In some pathogenic microbes, the response to oxidative stress is controlled by a SirTM/zinc-containing macrodomain (Zn-Macro) pair responsible for establishment and removal of the modification, respectively. Strikingly, however, the “catalytic loop” found in all other MacroD-type enzymes (also termed “loop 1”) is replaced with and extended loop containing the zinc-coordinating Cx(4)HxC motif, here termed the Zn-loop. To gain a closer understanding of the functional role of the 3α-bundle and coordinated Zn2+ ion, we solved structures from the three sub-branches of Zn-Macros namely from S. aureus (SauMacro), Methanobrevibacter oralis (MorMacro), and macrodomain-fused SirTM protein (Mfs1) from Fusarium oxysporum f.sp. cubense race 1 (Foc1Mfs1) in their apo form as well as of S. pyogenes (SpyMacro) and MorMacro bound to ADP-ribose (ADPr). In all structures, the Zn2+ ion is tetrahedrally coordinated with three metal-coordination residues within the Zn-loop, while the fourth coordination-contact is exchangeable and is provided by either ADPr, a water molecule, or a symmetry-related protomer within the crystal.

As before, SpyMacro WT from the extended operon background could remove the ADP-ribosyl modification. ADPr is tightly coordinated within the active site. Within the SpyMacro structure, the adenosine base is coordinated via an Asp92-adenine C6 amino group contact and Phe251 π-stacks with the base. The proximal ribose is rotated out of the active side and the C3′ position makes a conserved contact with Thr213. The C2′ OH moiety is solvent exposed, but the local environment makes it unlikely that a poly-ADPr chain could be accommodated, thus suggesting that Zn-Macros can only interact with terminal ADPr or mono-ADPr moieties. The ADPr diphosphate is primarily coordinated via residues of the—in MacroD-type enzymes—identified diphosphate-binding loop (also termed ‘loop 2’), which is located on the opposite side of the binding cleft relative to the catalytic loop. In SpyMacro, the ribose adopts a furanose ring with a 2′ endo pucker, while the distal ribose in MorMacro is in the linear form. Second, upon ADPr bind, the cavity is closed due to the reorientation of Phe216 (SpyMacro) into the active site to help fix the orientation of the distal ribose within the catalytic centre. We could observe an isostructural water molecule in our structures of SpyMacro and MorMacro in complex with ADPr and Asn-ADPr, respectively, thus suggesting that the Pα phosphate group could act as Lewis base in the reaction.

> GPMSMPSSFDLLGEMIGLLQTEQLTSSWACPLPNALTKRQDLWRALINQRPALPLSKDYLNLEDAYLDDWRASFVPVSVKDCQKTNYTSLFLYHGDIRYLAVDAIVNAANSELLGCFSPNHGCIDNAIHTFAGSRLRLACQAIMTEQGRKEAIGQAKLTSAYHLPASYIIHTVGPRITKGHHVSPIRADLLARCYRSSLDLAVKAGLTSLAFCSISTGEFGFPKKEAAQIAIKTVLKWQAEHPESKTLTTIFNTFTSEDKALYDTYLQKENNCE> PKVQTDPPSVPICDLYPNGVFPKGQECEYPPTQDGRTAAWRTTSEEKKALDQASEEIWNDFREAAEAHRQVRKYVMSWIKPGMTMIEICEKLEDCSRKLIKENGLNAGLAFPTGCSLNNCAAHYTPNAGDTTVLQYDDICKIDFGTHISGRIIDCAFTVTFNPKYDTLLKAVKDATNTGIKCAGIDVRLCDVGEAIQEVMESY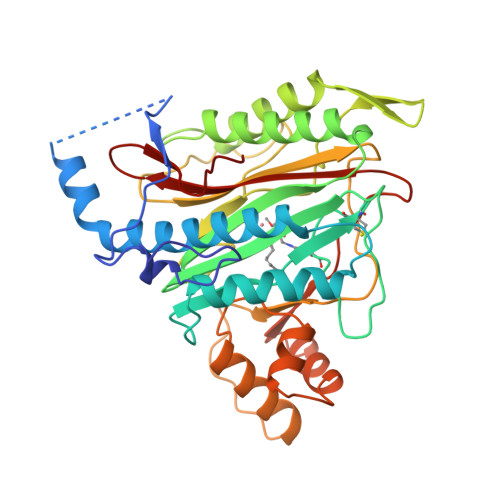EVEIDGKTYQVKPIRNLNGHSIGQYRIHAGKTVPIVKGGEATRMEEGEVYAIETFGSTGKGVVHDDMECSHYMKNFDVGHVPIRLPRTKHLLNVINENFGTLAFCRRWLDRLGESKYLMALKNLCDLGIVDPYPPLCDIKGSYTAQFEHTILLRPTCKEVVSRGDDY>[2x]SQVQNIPYAELEVGQKAEYTSSIAERDLQLFAAVSGDRNPVHLDAAYAATTQFKERIAHGMLSGALISAAIATVLPGPGTIYLGQTLRFTRP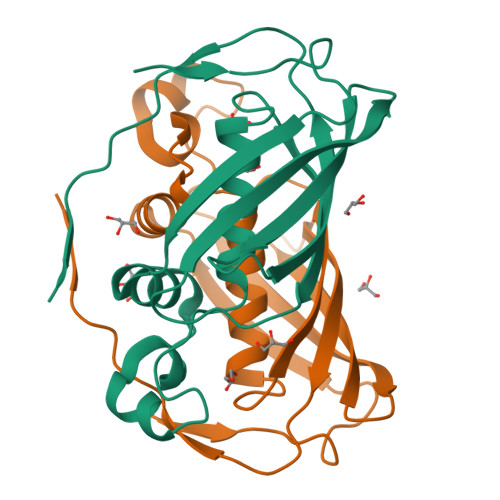VKLGDDLKVELEVLEKLPKNRVRMATRVFNQAGKQVVDGEAEIMAPEEKLSVELAELPPISIG> GSDGGTLAMLRGLSEDTLEQLYALGFNQYQAGKWDDAQKIFQALCMLDHYDARYFLGLGACRQSLGLYEQALQSYSYGALMDINEPRFPFHAAECHLQLGDLDGAESGFYSARALAAAQPAHEALAAR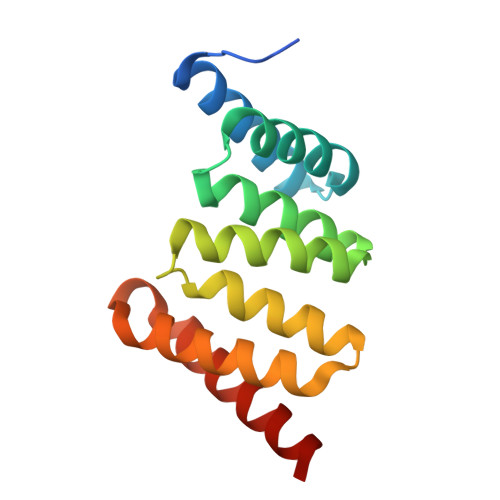AGAMLEAVTARKDR> QAQITGRPEWIWLALGTALMGLGTLYFLVKGMGVSDPDAKKFYAITTLVPAIAFTMYLSMLLGYGLTMVPFGGEQNPIYWARYADWLFTTPLLLLDLALLVDADQGTILALVGADGIMIGTGLVGALTKVYSYRFVWWAISTAAMLYILYVLFFGFTSKAESMRPEVASTFKVLRNVTVVLWSAYPV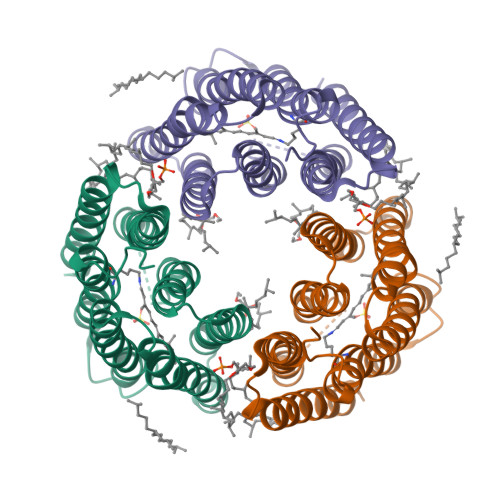VWLIGSEGAGIVPLNIETLLFMVLDVSAKVGFGLILLRSRAIFGEAEAPEPSAGDGAAATS>QQPGTSTPEVHPKLTTYKCTKSGGCVAQDTSVVLDWNYRWMHDANYNSCTVNGGVNTTLCPDEATCGKNCFIEGVDYAASGVTTSGSSLTMNQYMPSSSGGYSSVSPRLYLLDSDGEYVMLKLNGQELSFDVDLSALPCGENGSLYLSQMDENGGANQYNTAGANYGSGYCDAQCPVQTWRNGTLNTSHQGFCCNEMDILEGNSRANALTPHSCTATACDSAGCGFNPYGSGYKSYYGPGDTVDTSKTFTIITQFNTDNGSPSGNLVSITRKYQQNGVDIPSAQPGGDTISSCPSASAYGGLATMGKALSSGMVLVFSIWNDNSQYMN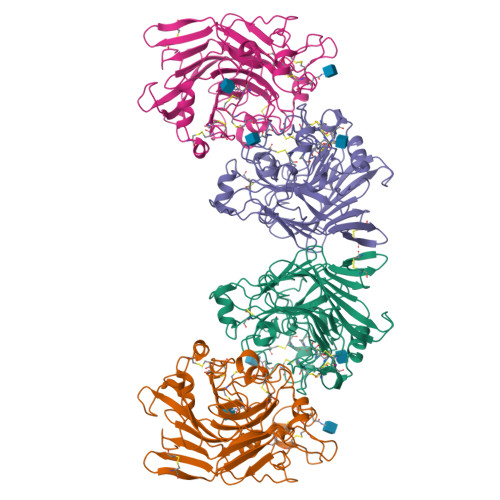WLDSGNAGPCSSTEGNPSNILANNPNTHVVFSNIRWGDIGSTT[2x]>DLSTSINPWFVTGFTDAEGSFMIHLEKNKDKWRVRPTFQIKLDIRDKSLLEEIKNYFNNTGSINTSNKECVYKV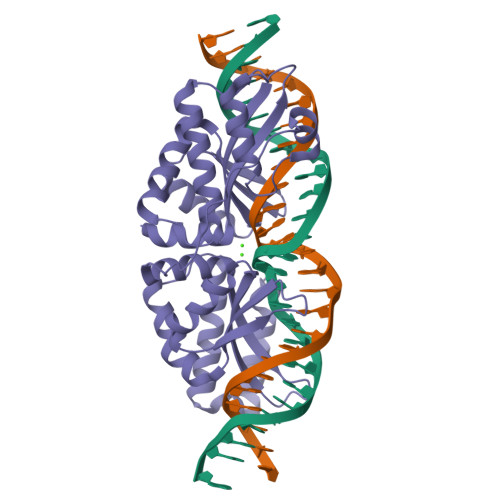RSLKDISIIISHFDKYNLITQKKADFELFKKIINKLNSQEHLSYEVGATVLQEIISIRASMNLGLSSSVKEDFPHIIPSNRPLIENMNIPHPEWMAGFVSGEGSFSVYTTSDDKYVSLSFRVSQHNKDKQLLKSFVDFFGCGGFNYHNKGNKAVIFVTRKFEDINDKIIPLFNEYKIKGVKYKDFKDWSKVAKMIESKSHLTTNGYKEICKIKENMNSYRKSSVN[2x]> MGSSHHHHHHSSGENLYFQGSHMID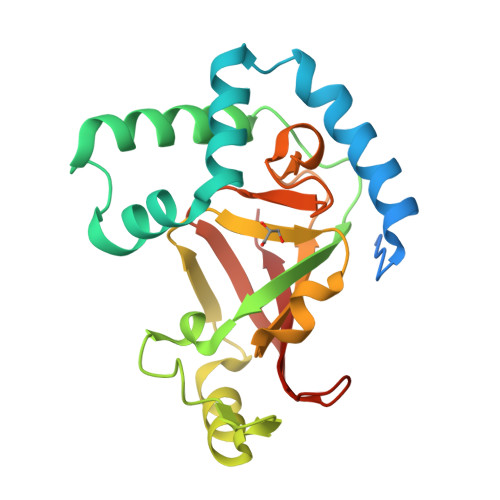FRIDKEKAKKWGKKEYSKWKSTLTEEEKRQITLYTRNASPINTYLREEGIGSKPDMDKKIELIDKALIKTKLKDSVTVYRGTDGIIFGKEFQNTLMNGNKVNGEVAKKIKKEFEGTMLLERGYLSTSLVNGTLFLARPVLIELKIPKGGNAGYVDPISYYPGQLEMLLPRDTKYYIDNIKIIVNGGSQRLKVEARVLS>ESSNKISCLPRVAQNLGYHYSPDLPGFCPIPKELAEHWPVVSNDRYPNCLQITLQQVCELSKPCSAGYMVGQSVFVQTPGVTSYWLTEWVDGKARALPDSLFSSGRFETNSRAFLDEAEEKFAAAHPHACLGEINKSTVGGSHFIFSQYLPPLLPADAVALVGASLAGKAAAAACSVVDVYAPSFEPYLHPETLSRV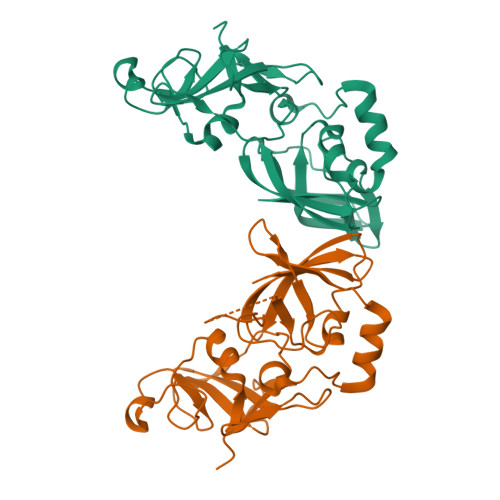YKIMIDFKPCRLMVWRNATFYVQE[6x]Bestrophin-1 (Best1) and bestrophin-2 (Best2) are two members of the bestrophin family of calcium (Ca2+)-activated chloride (Cl−) channels with critical involvement in ocular physiology and direct pathological relevance. The bestrophins are a family of Ca2+-activated anion channels consisting of four members (Best1–4) in mammals. The overall architecture of hBest1 and hBest2 resembles the pentameric assembly previously shown by KpBest, cBest1 and bBest2, and retains the two landmark permeation constrictions, the neck and aperture, in the ion conducting pathway. Ample electrophysiological evidence indicates that the neck and aperture serve as dual Ca2+-dependent channel “gates”, as disrupting either of them partially impairs Ca2+-dependence while disrupting both makes the channel completely Ca2+-independent.

Under both 1 μM and 5 mM Ca2+ conditions, most of the hBest1/hBest2 particles (~90–95%) were in a Ca2+-bound closed state, which is very similar to the Ca2+-unbound closed state. Strikingly, however, a small population of hBest1 and hBest2 particles exhibited a partially and fully open neck, respectively. A fully dilated neck is present in 6.3% and 12% of hBest2 particles exposed to 1 μM and 5 mM Ca2+ spike, respectively. This conformation resembles that of the previously solved cBest11–345 and cBest11–345-W287F19. Critical conformational changes take place at residues Y236, F282, F283, and W287, concomitant with the neck residues I76, F80 and F84 turning away from the ion conducting pore, drastically dilating the minimum radius of the neck from 0.8 Å to 4.5 Å and revealing a hydrophilic ion permeation pathway through the membrane. By comparing Ca2+-bound hBest2 in the closed and open states, we defined the structural changes coordinated with neck gating at residues 346–379. In the open state, by sharp contrast, residues 346–356 (yellow) and 369–379 (red) become fully disordered while moderate density remains for anchor residues 357–368 (blue), indicating diminished binding of this region to the channel periphery. Although the necks of hBest1 and hBest2 are formed by the same set of three residues (I76/F80/F84) as in cBest1 and bBest212,13, we discovered a partially open conformation of this gate in Ca2+-bound hBest1, in contrast to the fully open neck in hBest2 under the same conditions. Higher percentages of open neck particles were found in the 5 mM Ca2+ datasets compared to the 1 µM Ca2+ datasets and were all accompanied with the disordering of the AS, suggesting an influence of Ca2+ on the binding dynamics of the AS. Moreover, unlike the static apertures in previous studies, the apertures in hBest1 and hBest2 both display a distinct conformation in the presence of Ca2+, potentially representing a partially and fully open conformation of the aperture, respectively, as dilations take place at position 205, with an ion-like density captured at position 208.

>[5x]MTVTYTARVANARFGGFSQLLLLWRGSIYKLLWRELLCFLGFYMALSAAYRFVLTEGQKRYFEKLVIYCDQYASLIPVSFVLGFYVTLVVNRWWSQYLCMPLPDALMCVVAGTVHGRDDRGRLYRRTLMRYAGLSAVLILRSVSTAVFKRFPTIDHVVEAGFMTREERKKFENLNSSYNKYWVPCVWFSNLAAQARREGRIRDNSALKLLLEELNVFRGKCGMLFHYDWISVPLVYTQVVTIALYSYFLACLIGRQFLDPAQGYKDHDLDLCVPIFTLLQFFFYAGWLKVAEQLINPFGEDDDDFETNFLIDRNFQVSMLAVDEMYDDLAVLEKDLYWDAAEARAPYTAATVFQLRQPSFQGSTFDITLAKEDMQFQRLDGLDGPMGEAPGDFLQRLLPAGAGMVA1,2-DIOCTANOYL-SN-GLYCERO-3-PHOSPHATE | C19 H36 O8 P | 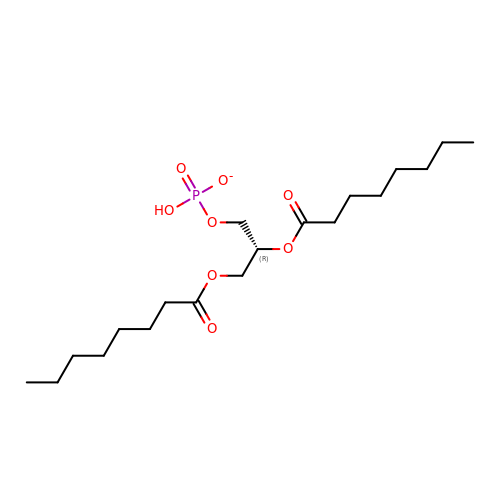XYSBQYUENLDGMI-QGZVFWFLSA-M(2~{S},3~{R})-8,9-dimethoxy-3-[2,4,5-tris(fluoranyl)phenyl]-2,3-dihydro-1~{H}-benzo[f]chromen-2-amine 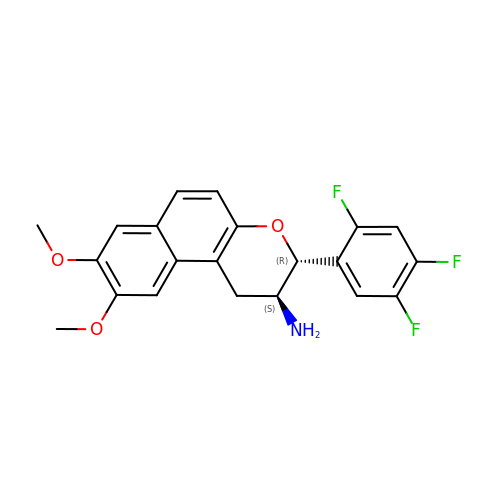| C21 H18 F3 N O3 | NXPAPTOHRVIGJL-LAUBAEHRSA-N S)-2-(5(((1,2-DIHYDRO-3-METHYL-1-OXOBENZO(F)QUINAZOLIN-9-YL)METHYL)AMINO)1-OXO-2-ISOINDOLINYL)GLUTARIC 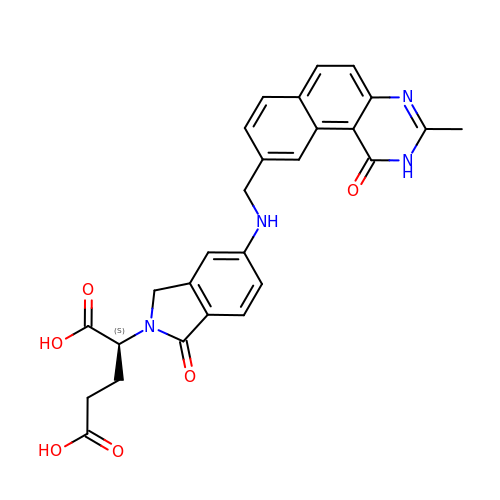ACID | C27 H24 N4 O6 | BRVFNEZMTRVUGW-QFIPXVFZSA-N> MDIQLFSKTPSVTVFDNRGLSVRDIAYRRHPDTPKVTEECITYHQFDFRGFLAQSLDPRLNHKEVTNFSYLTDLNGNIIYTQSVDAGNTLVLNDTEGRSVIAMTNISRGENGKDDLSLAVTRTFQYENAPLPGRPLSVTEQVNGENARITEHFVYAGNTPQEKNLNLAGQCVSYYDAAGLIQTDSVSLTGKPLSVSRKLLKNLDDTNILADWQGNDTSAWNSLLATEIYTTVTRTDAAGAVLTTIDAVGNQQRVAFDIAGQLSASWLTLKGGQEQVII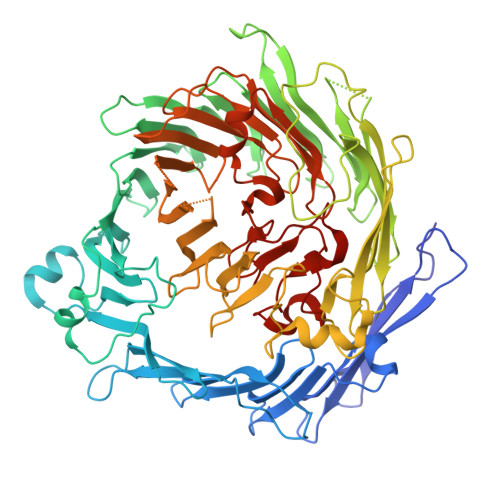KVLTYSAAGQKLREEGGNGVVTTYTYEAETQRLIGIKTERPNGHAAGAKVLQDLRYEYDPVGNVLSITNDAEETRFWRNQKVVPENAYRYDSLYQLVSASGREVAGAGQQGSDLPSPLVPLPSDSSVYTNYTRTYTYDSAGNLMRIRHSAPATNNNYTLNITVSERSNRGVMSSLTENPADVDALFTASGSQKCLQQGQSLIWTPRGELRTVLLVARGETADDSESYRYDGSSQRILKISSQQTNHSARVQRALYLPGLEWRTMTGGVAEAENLQVICIGEAGRAQVRVLHWESGKPDGIINDQIRWSYDNLTCSSGLEVDGDGLVISMEEYYPYGGTAVWAARSHIETAYKTVRYSGKERDATGLYYYGFRYYQPWAGRWLSADPAGTVDGLNLYRMVRNNPLRLTDPDGM>[2x]MAHHHHHHMELTEITPESLRLRPSHKERNVLITGAARGIGRAIAQAFVERSATVGICDLNLADVARTCEELNGLGLGRAVPIACDVSDYDALVAAIDDTGLVFDTVVNNAGISPKHNG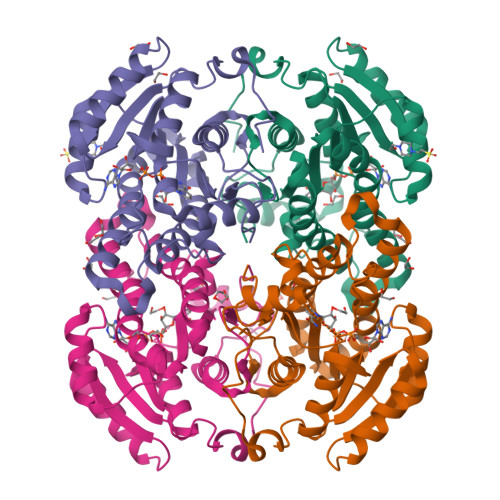VAHKVWEMAPDEWRRVVDVNLTGTFNTIRALTPGMVEARRGWIVNTSSVAGKTYSPIVACHYAATKSAIIGFTKHLAAELGPYSIRVNAMAPGRIATPMVAGVAPEVNAEQVKLTPMARLGQPAEVADVALWLTSTESSFVTGQTVDVAGGLYMA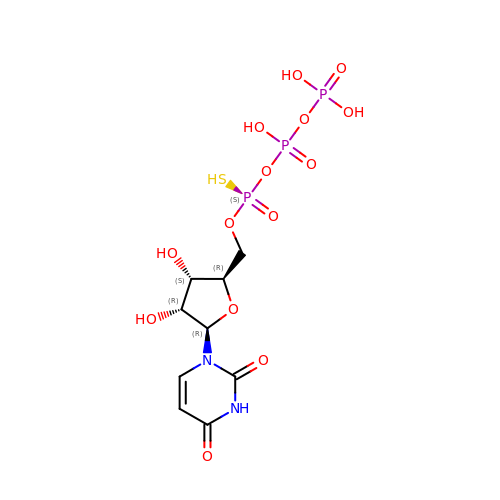[[(2~{R},3~{S},4~{R},5~{R})-5-[2,4-bis(oxidanylidene)pyrimidin-1-yl]-3,4-bis(oxidanyl)oxolan-2-yl]methoxy-sulfanyl-phosphoryl] phosphono hydrogen phosphate | C9 H15 N2 O14 P3 S | BWPNYQWDXHLOGU-KWWYXVLOSA-N>[2x]MAHHHHHHVDDDDKMNSDDNADGLIFSPLPQNKNTVVRHYSNEQEMPNLSQMAQRTIDFPTQIVRVSGNLTGLELSCDDVENEIDQVFSKKISPNLFTYNTYVSCGYDVNDPEQHATNFSIQSYFDPLTDNAVDYLKSYLKEYNGYNLFNTTTLQIENAKGIIVSMNLNAGLKSNPDKTPFTLYRQDRNNFYFKSNFDVRKELISDIYQRFYSNDPDMILPFFDKWIFSYAGSVYYSILMASNYLELQPERIFVMENEGDIFVSDLRYYFANLCMKRNPNKHCL

L. pneumophila also expresses a type II secretion system (T2SS). The Legionella T2SS exports at least 25 proteins. In summary, using a combined cellular, structural, biophysical and biochemical approach we have provided a characterization of three novel type II secreted substrates, NttA, NttC and NttE, that are required for infection of several species of amoeba. We also report the X-ray crystal structures of NttE and NttC, the solution nuclear magnetic resonance (NMR) structure of NttA and dynamic analyses for each substrate using complementary biophysical techniques.

Previous proteomic analysis of culture supernatants from wild-type L. pneumophila 130b strain (a clinical isolate) and a T2SS (lspF) mutant identified NttE, a 288-amino acid protein encoded by the lpw02811 ORF (lpg0189 in strain Philadelphia-1; lpp0250 in strain Paris; lpl0249 in strain Lens), as a secreted substrate of the L. pneumophila T2SS. Crystals of NttE were obtained at pH 6.5 and the structure was determined using selenium single-wavelength anomalous dispersion (Se-SAD) phasing with electron density maps refined to 2.2 Å. The final model contains two molecules in the asymmetric unit and all residues could be built except for the N-terminal His6 tags and the NttE residues Asn1 to Ala6. Each NttE protomer is formed of two domains, with the N-terminal domain (residues T20 to N143) composed of 7 α-helices and 3 β-strands, and the C-terminal domain (residues D7 to F11 and G146 to L269) formed from 5 α-helices and 4 β-strands. Two disulfide bonds are present in each chain of NttE, one in the N-terminal domain between Cys62 and Cys90, and another in the C-terminal domain between Cys259 and Cys268. The NttE dimer is mainly stabilized through β-sheet interactions provided by the C-terminal domain and the presence of this dimer in the asymmetric unit strongly indicates that NttE is a dimer in solution. The NttE α1 helix mediates hydrophobic interactions with the α4 helix in the C-terminal domain, and it appears that small changes in this interface results in large changes in the orientation of the N-terminal region. However, analysis of all known sequences of NttE homologs from Legionella species and A. siphonis revealed a conservation hotspot at the interface of the N- and C-terminal domains, positioned on the “top” face of the NttE dimer. Comparison of the two models with lowest χ2 values with the crystal structure of NttE-130b highlighted significant variability in the positioning of the N-terminal domains, although in all models the β1 strand remained tethered to the C-terminal domain. Together these data indicate that the N-terminal domains of NttE are mobile and this may be important for its function in modifying the bacterial cell surface and/or during intracellular infection.>[2x]MEDVAGNYDDTFGDVQKQIVNYFTYKAVRTVLHQLYEMNPPQYTWFYNHIITNRPTDGKRFLRALGKESQELAERVMITRLHLYGKWIKKADHGKIYQEISD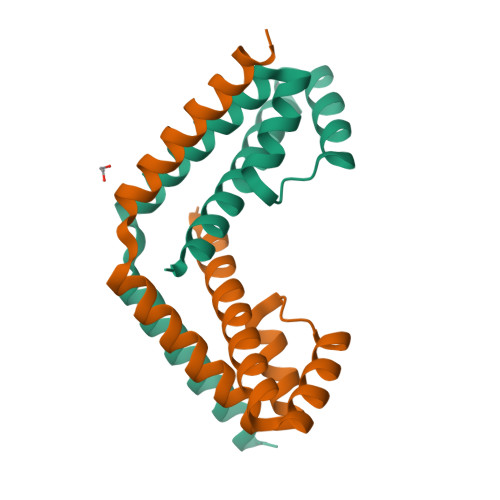ENLALMRERLMETVIWPSDDTNSR> GSMSAKDERA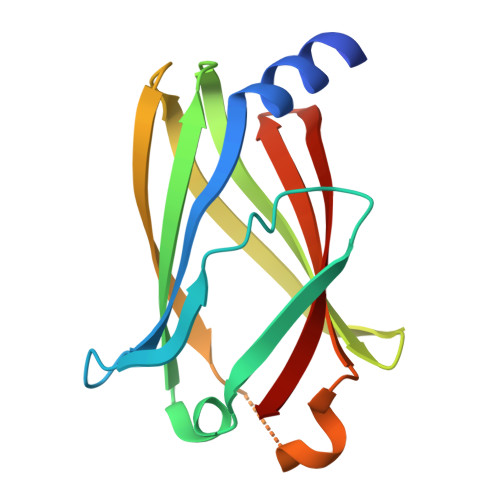REILRGFKLNWMNLRDAETGKILWQGTEDLSVPGVEHEARVPKKILKCKAVSRELNFSSTEQMEKFRLEQKVYFKGQCLEEWFFEFGFVIPNSTNTWQSLIEAAPESQMMPASVLTGNVIIETKFFDDDLLVSTSRVRLFYV> TPE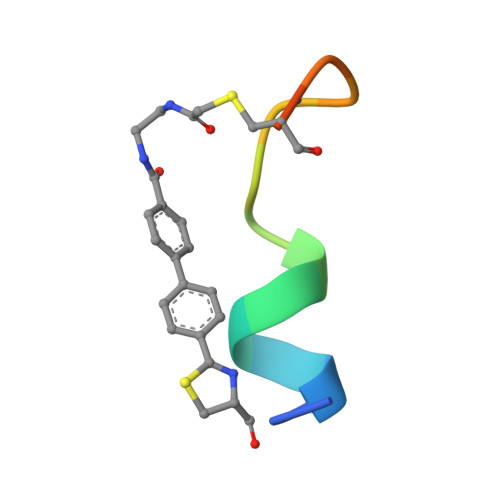WASTLRPECXXP>[60x]SIKYIFKKTDTLPRSVIGNVLRTTGPDTTVYSLPGHTPVNPFTLTAVSRLPVPRKGNAGTTKTTLSLRREVTINKGTDQEKIVPMIARIETSVPVGVSQDDFKAMIEGLACPLLL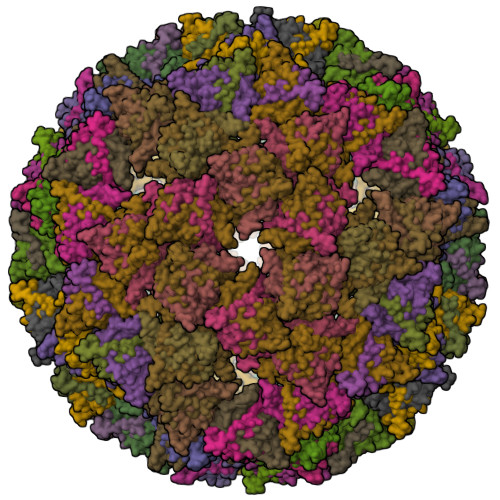DEIHVNDLFLSGLPIATTDVPDNEPLPPALL The first enzyme in the pathway, peptide O-xylosyltransferase (XT, EC 2.4.2.26), catalyzes the transfer of xylose from uridine diphosphate (UDP)-α-D-xylose onto serine and thus determines the site(s) of GAG attachment on the core protein. XT1 and XT2 are type II transmembrane proteins consisting of a short amino-terminal region facing the cytosol, a single transmembrane helix, a stem region required for Golgi localization (Schön et al., 2006), a catalytic GT-A domain (Lairson et al., 2008, Müller et al., 2006), and a unique C-terminal domain of unknown function, termed “Xylo_C” in the Pfam database (Finn et al., 2008). XT1 has a two-lobed structure, with one lobe comprising the catalytic GT-A domain and the other comprising the Xylo_C domain. To better understand the initial step of GAG biosynthesis, we have determined crystal structures of human XT1 complexed with UDP-xylose and various PG-derived acceptor peptides.

To visualize how the different amino acid substitutions are accommodated in the peptide binding cleft, we selected five variants of the bikunin-derived peptide for structure analysis (peptides 3–7). Three bikunin variants bound identically to the wild-type peptide: peptide 3 (proline at position −3), peptide 5 (alanine at position +1), and peptide 7 (proline at position +3). Proline can be accommodated at positions −3 and +3, where the wild-type peptide naturally adopts a backbone conformation favorable for proline.

> APLVHHHHHHALDENLYFQGALADVSRPPHARKTGGSSPETKYDQPPKCDISGKEAISALSRAKSKHCRQEIGETYCRHKLGLLMPEKVTRFCPLEGKANKNVQWDEDSVEYMPANPVRIAFVLVVHGRASRQLQRMFKAIYHKDHFYYIHVDKRSNYLHRQVLQVSRQYSNVRVTPWRMATIWGGASLLSTYLQSMRDLLEMTDWPWDFFINLSAADYPIRTNDQLVAFLSRYRDMNFLKSHGRDNARFIRKQGLDRLFLECDAHMWRLGDRRIPEGIAVDGGSDWFLLNRRFVEYVTFSTDDLVTKMKQFYSYTLLPAESFFHTVLENSPHCDTMVDNNLRITNWNRKLGCKCQYKHIVDWCGCSPNDFKPQDFHRFQQTARPTFFARKFEAVVNQEIIGQLDYYLYGNYPAGTPGLRSYWENVYDEPDGIHSLSDVTLTLYHSFARLGLRRAETSLHTDGENSCRYYPMGHPASVHLYFLADRFQGFLIKHHATNLAVSKLETLETWVMPKKVFKIASPPSDFGRLQFSEVGTDWDAKERLFRNFGGLLGPMDEPVGMQKWGKGPNVTVTVIWVDPVNVIAATYDILIESTAEFTHYKPPLNLPLRPGVWTVKILHHWVPVAETKFLVAPLTFSNRQPIKPEEALKLHNGPLRNAYMEQSFQSLNPVLSLPINPAQVEQARRNAASTGTALEGWLDSLVGGMWTAMDICATGPTACPVMQTCSQTAWSSFSPDPKSELGAVKPDGRLR;> QEPEGSGGGQG> IKDILRRPVLLFNHVELDPDYTGFFIPIMPPSRMMQYKSGDKETSFQRLIGRTPQAAIMNLFRFWRGSLRYTIIIHSTDGHPIYVTHVPHTGNRVYGLMKVNNLHEYTKVPIFGCGLTTEMIIPSVNPSICVE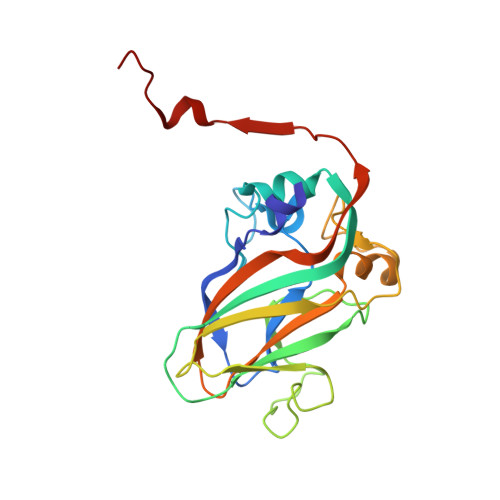VPFDTENNWAVTFDEDAQRNYSWRDKGDTVTGHLVVTPVVSVYMSVWVEAGDDFEVSNFYGPPSVKTNDWNYAFSDEH> IAGGEAITTGGSRCSLGFNVSVNGVAHALTAGHCTNISASWSIGTRTGTSFPNNDYGIIRHSNPAAA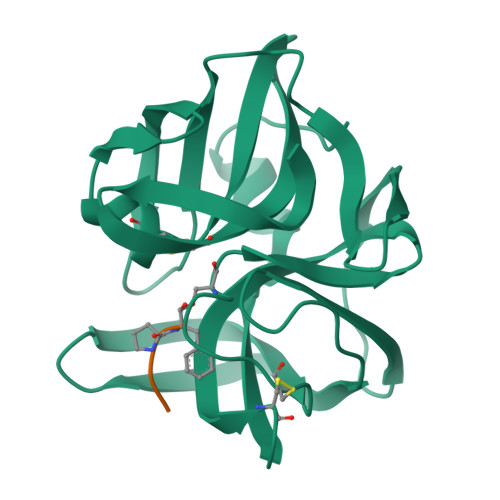DGRVYLYNGSYQDITTAGNAFVGQAVQRSGSTTGLRSGSVTGLNATVNYGSSGIVYGMIQTNVCAQPGDSGGSLFAGSTALGLTSGGSGNCRTGGTTFYQPVTEALSAYGATVL;> XPAPF> TLTEDLDAPQDTGNIENGAADNSPQPRTTFDYTGNPLPPDTKLENFFSFYRLLPMGGSGAPSLSFPADEGTIIPLNPINWLKGADVSGIAAMLSCFTYIAADLRITLRFSNPNDNPATMLVAFAPPGATIPLKPTRQMLSNFYMAEVPVSAATSTMVSFSIPYTSPLSAIPTSYFGWEDWSGTNFGQLSSGSWGNLMLIPSLSVDSAIPFDFQLSCWVAFGNFKAWVPRPPPPLPPLPTPAANAERTVAVIKQ;> GNSVTNIYGNGNNVTTDVGANGWAPTVSTGLGDGPVSASADSLPGRSGGASSEKTHTVSGSSNKVGSRFSKWWEPAAARASESATDSAIEGIDAAGKAASKAITRKLDRPAAPSSTANPQPSLIA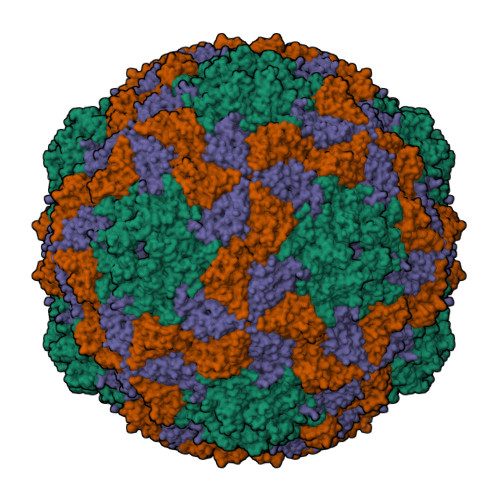LNPSATQSGNASILTGSTAPSLLAYPTATPVPLPNPDEPSQPGPSGDRTWLLDTVTWSQEFTRGWNIAGSNGMQWTGLESLIFPVSTDTNWTSTSSPTAYPLPFSFVRAYPDSSWAAMYNTHSMWNCGWRVQVTVNGSQFHAGALILYMVPEATTHAIQTARDNAGFVFPYVILNLYESNTATIEVPYISPTPNTSSGLHAPWTFYLQVLSPLNPPPSLPTSLSCSIYVTPVDSSFHGLRYLAPQ;> HWKTRAVPGAGTFGSAVAGQELPLCGVRAYYPPNAYIPAQVRDWLEFAHRPGLMATVPWTMADEPAERLGIFPVSPSAIAGTGAPISYVISLFSQWRGELAAHLLFTGSAQHYGRLVVCYTPAAPQPPSTMQEAMRGTYTVWDVNAASTLEFTIPFISNSYWKTVDVNNPDALLSTTGYVSIWVQNPLVGPHTAPASALVQAFISAGESFNVRLMQNPALTSQ> KKGQSTSRHKKLMFKT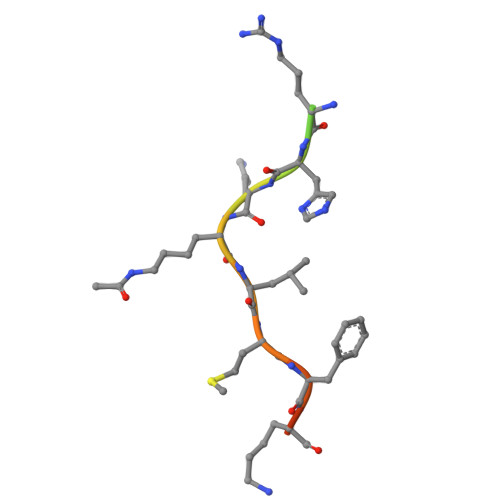EG>MGSSHHHHHHSSGLVPRGSMANYTEKFAAWSVICLTDHTFLDENGTEDDIRELCNESVKTCPFAAAVCVYPKFVKFINEKIKQEINPFKPKIACVINFPYGTDSMEKVLNDTEKALDDGADEIDLVINYKKIIENTDEGLKEATKLTQSVKKLLTNKILKVIIE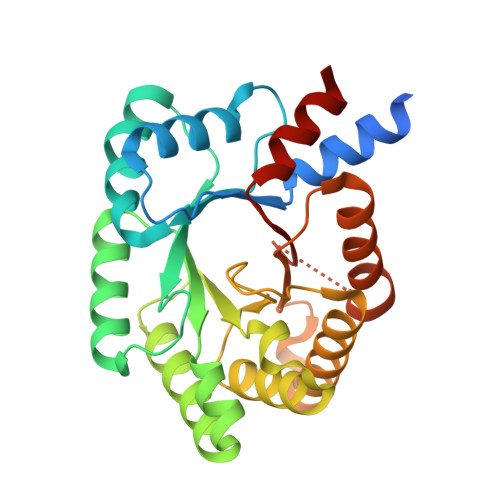VGELKTEDLIIKTTLAVLNGNADFIKTSTGKVQINATPSSVEYIIKAIKEYIKNNPEKNNKIGLKVSGGISDLNTASHYILLARRFLSSLACHPDNFRIGSSSLVIKLRKVISQCPL[2x]>[2x]GHMINYPLASSTWD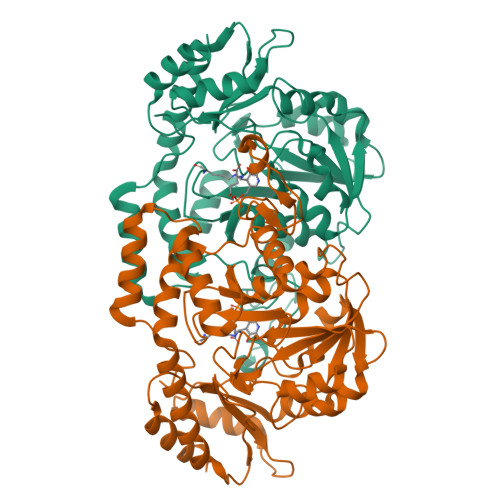DLEYKAIQSVLDSKMFTMGEYVKQYETQFAKTFGSKYAVMVSSGSTANLLMIAALFFTKKPRLKKGDEIIVPAVSWSTTYYPLQQYGLRVKFVDIDINTLNIDIESLKEAVTDSTKAILTVNLLGNPNNFDEINKIIGGRDIILLEDNCESMGATFNNKCAGTFGLMGTFSSFYSKHIATMEGGCIVTDDEEIYHILLCIRAHGWTRNLPKKNKVTGVKSDDQFEESFKFVLPGYNVRPLEMSGAIGIEQLKKLPRFISVRRKNAEYFLDKFKDHPYLDVQQETGESSWFGFSFIIKKDSGVIRKQLVENLNSAGIECRPIVTGNFLKNTDVLKYFDYTVHNNVDNAEYLDKNGLFVGNHQIELFDEIDYLREVLK>MKHGIYYAYWEQEWEADYKYYIEKVAKLGFDILEIAASPLPFYSDIQINELKACAHGNGITLTVGHGPSAEQNLSSPDPDIRKNAKAFYTDLLKRLYKLDVHLIGGALYSYWPIDYTKTIDKKGDWERSVESVREVAKVAEACGVDFCLEVLNRFENYLINTAQEGVDFVKQVDHNNVKVMLDTFHMNIEEDSIGGAIRTAGSYLGHLHTGECNRKVPGRGRIPWVEIGEALADIGYNGSVVMEPFVRMGGTVGSNI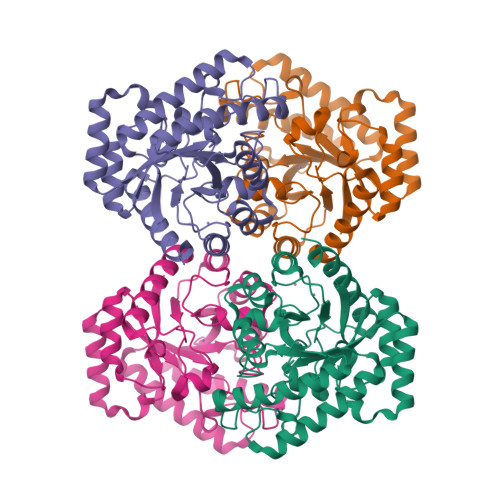KVWRDISNGADEKMLDREAQAALDFSRYVLECHKHS[4x]>MKVFEFEVGKGFLLRLDYGKDLVRQIEEFLEEKGIHAAHISAIGAVRSAVIGYYDQEK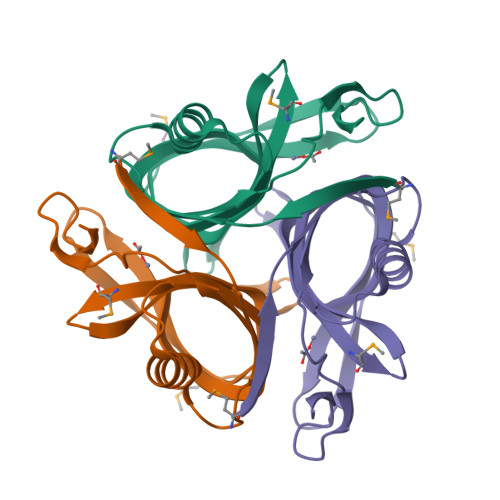KEYVKKELMEPLEILSLSGNVSMKDSKPFCHIHVLLGKDGEVYGGHLFSAEVFACEVFVLPLSGEAPERAFDEQTGLFLWLEHHHHHH[3x]>[2x]GPLGSARMKQFKDMLLERGVSAFSTWEKELHKI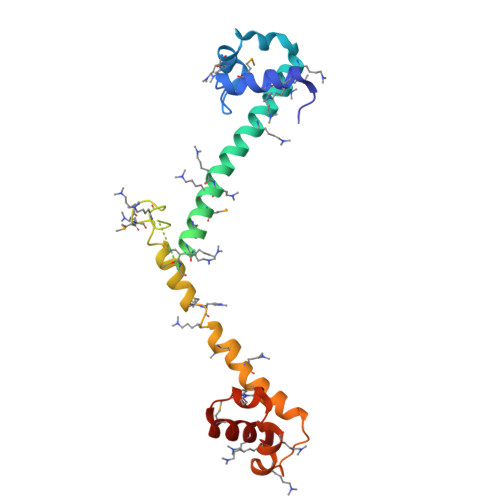VFDPRYLLLNPKERKQVFDQYVKTRAEEERREKKNKIMQAKEDFKKMMEEAKFNPRATFSEFAAKHAKDSRFKAIEKMKDREALFNEFVAAARKKEKEDSKTRGEKIKSDFFELLSNHHLDSQSRWSKVKDKVESDPRYKAVDSSSMREDLFKQYIE> MNARSTGQHPARYPGAAAGEPTLDSWQEPPHNRWAFAHLGEMVPSAAVSRRPVNAPGHALARLGAIAAQLPDLEQRLEQTYTDAFLVLRGTEVVAEYYRAGFAPDDRHLLMAVSKSLCGTVVGALVDEGRIDPAQPVTEYVPELAGSVYDGPSVLQVLDMQISIDYNEDYVDPASEVQTHGRSAGWRTRRHGDPADTYEFLTTLRGDGSTGEFQYCSANTDVLAWIVERVTGLRYVEALSTYLWAKLDADRDATITVDTTGFGFAHGGVSCTARDLARVGRMMLDGGVAPGGRVVSEDWVRRVLAGGSHEAMTDKGFTNTFPDGSYTRQWWCTGNERGNVSGIGIHGQN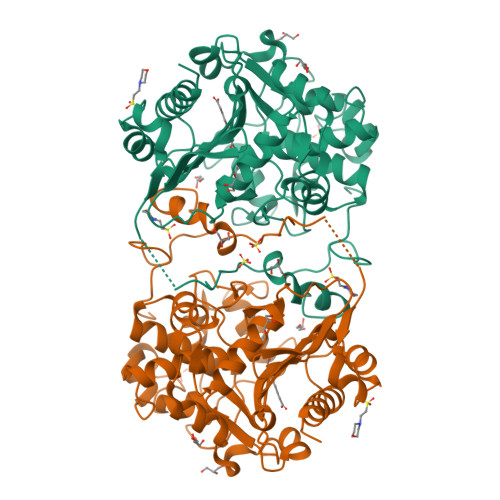LWLDPLTDSVIVKLSSWPDPYTEHWHRLQNGILLDVSRALDAV> MAQALPWLLLWMGAGVLPAHGTQHGIRLPLRSGLGGAPLGLRLPRETDEEPEEPGRRGSFVEMVDNLRGKSGQGYYVEMTVGSPPQTLNILVDTGSSNFAVGAAPHPFLHRYYQRQLSSTYRDLRKGVYVPYTQGKWEGELGTDLVSIPHGPNVTVRANIAAITESDKFFINGSNWEGILGLAYAEIARPDDSLEPFFDSLVKQTHVPNLFSLQLCGAGFPLNQSEVLASVGGSMIIGGIDHSLYTGSLWYTPIRREWYYEVIIVRVEINGQDLKMDCKEYNYDKSIVDSGTTNLRLPKKVFEAAVKSIKAASSTEKFPDGFWLGEQLVCWQAGTTPWNIFPVISLYLMGEVTNQSFRITILPQQY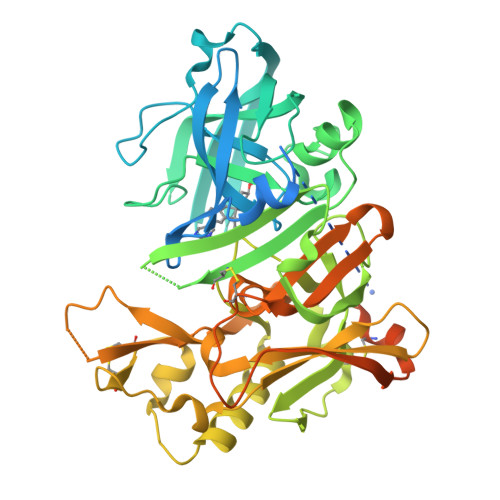LRPVEDVATSQDDCYKFAISQSSTGTVMGAVIMEGFYVVFDRARKRIGFAVSACHVHDEFRTAAVEGPFVTDLMEDCGYNIPQTDESTLMTIAYVMAAICALFMLPLCLMVCQWRCLRCLRQQHDDFADDISLLK1-{(1R,2S)-1-[2-(2,3,-DICHLOROPHENYL)ETHYL]-2-HYDROXYPROPYL}-1H-IMIDAZOLE-4-CARBOXAMIDE | 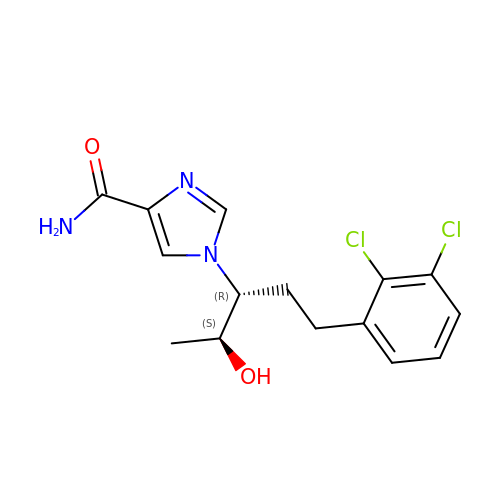C15 H17 Cl2 N3 O2 | HCJYSIGJDKNVRU-TVQRCGJNSA-N>[3x]MPACC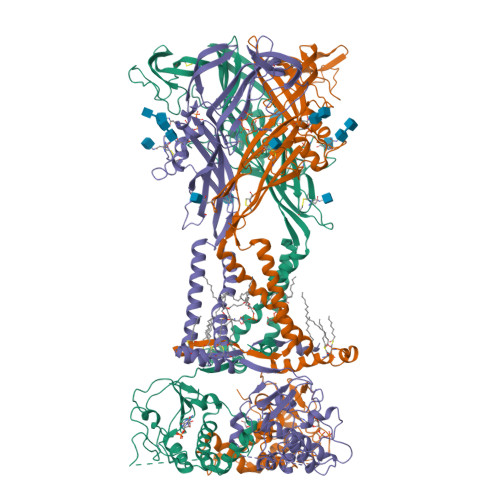SWNDVFQYETNKVTRIQSVNYGTIKWILHMTVFSYVSFALMSDKLYQRKEPLISSVHTKVKGVAEVTENVTEGGVTKLVHGIFDTADYTLPLQGNSFFVMTNYLKSEGQEQKLCPEYPSRGKQCHSDQGCIKGWMDPQSKGIQTGRCIPYDQKRKTCEIFAWCPAEEGKEAPRPALLRSAENFTVLIKNNIDFPGHNYTTRNILPGMNISCTFHKTWNPQCPIFRLGDIFQEIGENFTEVAVQGGIMGIEIYWDCNLDSWSHRCQPKYSFRRLDDKYTNESLFPGYNFRYAKYYKENGMEKRTLIKAFGVRFDILVFGTGGKFDIIQLVVYIGSTLSYFGLATVCIDLIINTYASTCCRSRVYPSCKCCEPCAVNEYYYRKKCEPIVEPKPTLKYVSFVDEPHIWMVDQQLLGKSLQDVKGQEVPRPQTDFLELSRLSLSLHHSPPIPGQPEEMQLLQIEAVPRSRDSPDWCQCGNCLPSQLPENRRALEELCCRRKPGQCITTSELFSKIVLSREALQLLLLYQEPLLALEGEAINSKLRHCAYRSYATWRFVSQDMADFAILPSCCRWKIRKEFPKTQGQYSGFKYPYSNSAVDAGLEVLFQ>MGSDKIHHHHHHMKIDILDKGFVELVDVMGNDLSAVRAARVSFDMGLKDEERDRHLIEYLMKHGHETPFEHIVFTFHVKAPIFVARQWFRHRIASYNELSGAYSKLSYEFYIPSPERLEGYKTTIPPERVTEKISEIVDKAYRTYLELIESGVPREVARIVLPLNLYTRFFWTVNARSLMNFLNLRADSH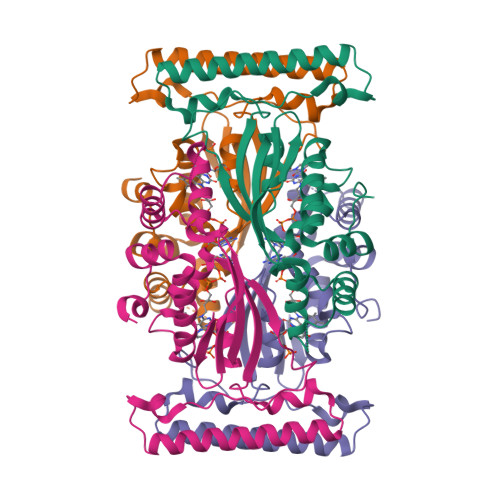AQWEIQQYALAIARIFKEKCPWTFEAFLKYAYKGDILKEVQV[4x]> MGSSHHHHHHSQDPMTVTANQVLRPRGPQIERLTDNRAKVVIEPLERGYGHTLGNALRRVLLSSIPGFAITEVEIDGVLHEYTTVEGLQEDVLDVLLNLKDVAIRMHSGDSATLSLSKQGPGTVTAADIRTDHNVEIINGDHVICHLTKDTALNMRLKIERGFGYQPAAARRRPDEETRTIGRLMLDASFSPVRRVAYAVEAARVEQRTDLDKLVIDIETNGTIDAEEAVRTAADILSDQ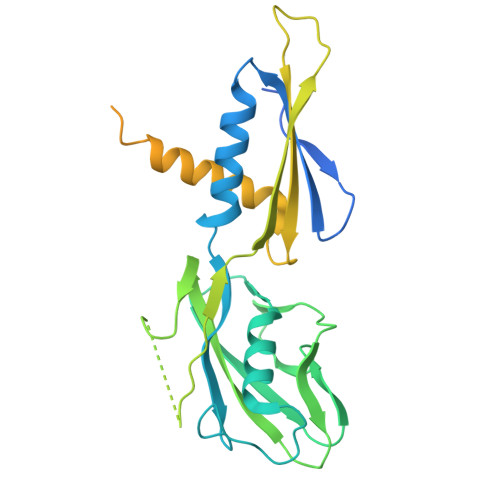LSVFGDFTHRDRGAAKPAASGVDPVLLRPIDDLELTVRSANCLKAESIYYIGDLIQKTEVELLKTPNLGKKSLTEIKEVLAQRGLALGMKLENWPPAGVAQHGMLG>GSHMSWVQLAGHTGSFKAAGTSGLILKRCSEPERYCLARLMADALRGCVPAFHGVVERDGESYLQLQDLLDGFDGPCVLDCKMGVRTYLEEELTKARERPKLRKDMYKKMLAVDPEAPTEEEHAQRAVTKPRYMQWREGISSSTTLGFRIEGIKKADGSCSTDFKTTRSREQVLRVFEEFVQGDEEVLRRYLNRLQQIRDTLEVSEFFRRHEVIGSSLLFVHDHCHRAGVWLIDFGKTTPLPDGQILDHRRPWEEGNREDGYLLGLDNLIGILASLAER[2x]

InsP3 3-kinase, a highly specific enzyme binding InsP3 in just one mode, phosphorylates InsP3 specifically at its secondary 3-hydroxyl group to generate a tetrakisphosphate. The structure of the IP3K kinase domain (IP3K-KD) revealed that the inositol polyphosphate kinase (IPK) family conserves the protein kinase (PK) fold organization in two lobes, the N- and C-lobes, binding the ATP in between them in a similar way. However, they present a third lobe, the IP-lobe inserted into the C-lobe, which accounts for most of the interactions with the inositide substrate. Summarizing, IP3K substrate recognition entails close interactions with the three phosphates in positions 1, 4 and 5 of the InsP or of the corresponding carbohydrate-based analogues.

We observed that this depends on the nature of the substituent at pseudo 2-position of the inositol ring. Thus, an axial OH in this position, (InsP3 and compound 4-s), forces the ligand to fit in the InsP3-site. All InsP3 (or InsP4) isomers (compounds 1–4) retain the ability to stabilize the enzyme significantly. Finally, the presence of two axial -OH groups (4-s) constitutes the least stabilizing isomers in this group.>[9x]MKQKVHSVSYLAKAEFEYKNGVYDLVALPTGAEVIKISLEVVGLPTAGHVSVGFKDESKKNYSSILTLPVNETSGVVTKDYTVKSDKIVAAEVKDALAEGSDGRPVKCVLRALYFLPSVIEVEY;>MLEKLNNINFNNISNNPNLGIEVGREIQNASWVKSPFFSITGTGADRGVRLFSVASQQPFRPRIKAQLTGSGVSGNTDFEANYDNLEI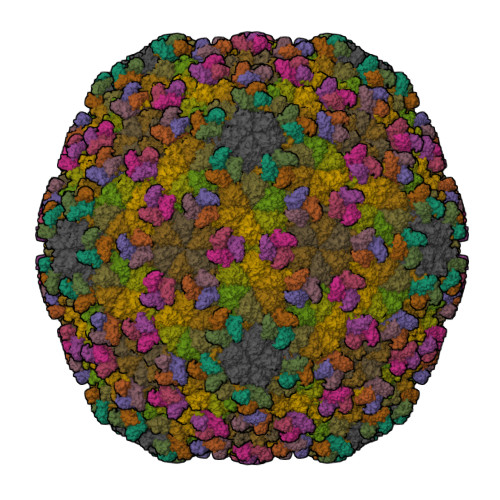LSQTIYPDAFGNSLRSKIKAYSELERIDFIKESVDSLTTWMNEERDKRIVASLTNDFTNYLYNAAMNVATIRKAIFHARNGLKADNSKAFPIKPIRATMQSVGNVVVQNTSYIILLDSYQANQLKADSEFKELRKLYAFAGEDKGMLYSGLLGVIDNCPVIDAGVWNKLNVGMPNSSISDSDFTRYLNKANVSNIVTPMQLKEKLNQEKLNQEKLNQEKLKNKDISIGCLIGASAVLLAGSKETRFYIDETVDAGRKSLVGVDCLLGVSKARYQSTDGVVTPYDNQDYAVIGLVSNME[9x]> XDPAWNHCEYAAFVC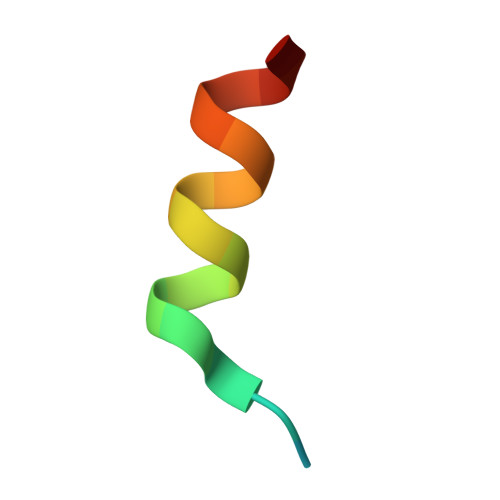SEVX As mycobacteria lack DNA mismatch repair, the only process that can ensure low levels of mutation during DNA replication is the replicative DNA polymerase and the associated proofreading exonuclease. Instead, the Mtb replicative DNA polymerase DnaE1 uses a PHP-exonuclease that is intrinsic to the protein itself. Recently, we have shown that in mycobacteria, the PHP domain is the essential replicative exonuclease and that the DnaQ-like DEDD exonuclease in contrast is dispensable. In addition, we have shown that the PHP domain of Mtb DnaE1 is a potential target for new antibiotics as its inactivation leads to strongly decreased growth rates and renders mycobacteria sensitive to nucleotide analogs that are used in antiviral therapy.

The crystal structure of M. tuberculosis DnaE1 was determined by X-ray crystallography to 2.8 Å resolution. To promote crystallization, the C-terminal region was removed (residues 942−1187), analogous to the structure of E. coli DNA Pol IIIα12. The final structure contains residues 1–933 and can be divided into four domains: the N-terminal PHP domain (residues 1–300), the thumb domain (residues 451–542), the palm domain (residues 301–450 and 543–591), and fingers domain (residues 592–933). The only exception is a loop in the thumb domain (residues 501–508) that is poorly defined in the density, most likely due to the absence of DNA. The polymerase active site, comprising aspartates 421, 423, and 587, is located at the bottom of the deep cleft between the thumb, palm, and fingers domain. On the other side of the thumb domain, ~40 Å away from the polymerase active site, is the exonuclease active site. It is located in the center of the PHP domain and consists of nine conserved residues that coordinate three metals. The coordinating residues comprise five histidines, three aspartates/glutamates, and one cysteine. The presence of a strong anomalous difference map around the metals at the high energy, but not the low energy data set, unambiguously identifies all three metals as zinc. Unique to the Mtb PHP domain is a long, 29-residue loop (residues 77–105) adjacent to the PHP active site.

> GSSFVHLHNHTEYSMLDGAAKITPMLAEVERLGMPAVGMTDHGNMFGASEFYNSATKAGIKPIIGVEAYIAPGSRFDTRRILWGDPSQKADDVSGSGSYTHLTMMAENATGLRNLFKLSSHASFEGQLSKWSRMDAELIAEHAEGIIITTGCPSGEVQTRLRLGQDREALEAAAKWREIVGPDNYFLELMDHGLTIERRVRDGLLEIGRALNIPPLATNDCHYVTRDAAHNHEALLCVQTGKTLSDPNRFKFDGDGYYLKSAAEMRQIWDDEVPGACDSTLLIAERVQSYADVWTPRDRMPVFPVPDGHDQASWLRHEVDAGLRRRFPAGPPDGYRERAAYEIDVICSKGFPSYFLIVADLISYARSAGIRVGPGRGSAAGSLVAYALGITDIDPIPHGLLFERFLNPERTSMPDIDIDFDDRRRGEMVRYAADKWGHDRVAQVITFGTIKTKAALKDSARIHYGQPGFAIADRITKALPPAIMAKDIPLSGITDPSHERYKEAAEVRGLIETDPDVRTIYQTARGLEGLIRNAGVHACAVIMSSEPLTEAIPLWKRPQDGAIITGWDYPACEAIGLLKMDFLGLRNLTIIGDAIDNVRANRGIDLDLESVPLDDKATYELLGRGDTLGVFQLDGGPMRDLLRRMQPTGFEDVVAVIALYRPGPMGMNAHNDYADRKNNRQAIKPIHPELEEPLREILAETYGLIVYQEQIMRIAQKVASYSLARADILRKAMGKKKREVLEKEFEGFSDGMQANGFSPAAIKALWDTILPFADYAFNKSHAAGYGMVSYWTAYLKANYPAEYMAGLLTSVGDDKDKAAVYLADCRKLGITVLPPDVNESGLNFASVGQDIRYGLGAVRNVGANVVGSLLQTRNDKGKFTDFSDYLNKIDISACNKKVTESLIKAGAFDSLGHARKGLFLVHSDAVD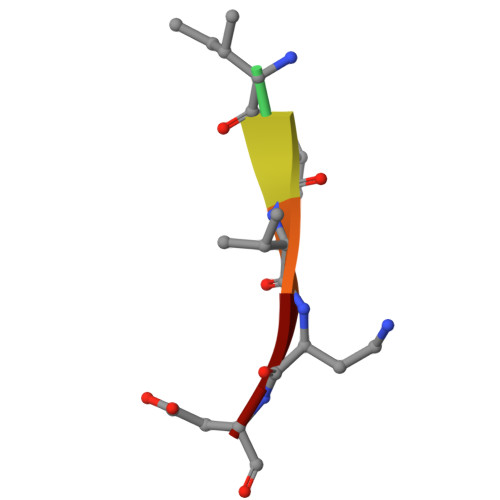> XITVAD>MGNAKTRRRERRAEKQAQWKAANAGAGAGAMATPHFDYIASVVSKGLANLSLELRKPVTFDIITADTLEQAIERAGTKHGNKGWEAALSAIEMANLFKS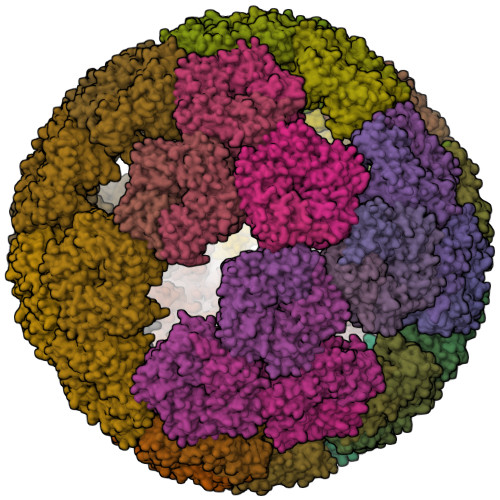LRGTGHHHHHHGSSMEIYEGKLTAEGLRFGIVASRFNHALVDRLVEGAIDCIVRHGGREEDITLVRVPGSWEIPVAAGELARKEDIDAVIAFGDLIRG[180x]> GSDELYRQSLEIISRYLREQATGAKDTKPMGRSGATSRKALETLRRVGDGVQRNHETAFQGMLRKLDIKNEDDVKSLSRVMIHVFSDGVTNWGRIVTLISFGAFVAKHLKTINQESCIEPLAESITDVLVRTKRDWLVKQRGWDG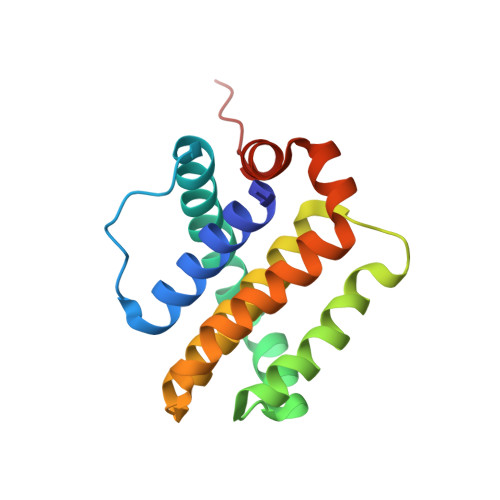FVEFFHVEDLE N,1-dimethyl-N-(propan-2-yl)-1H-pyrazolo[3,4-d]pyrimidin-4-amine | C10 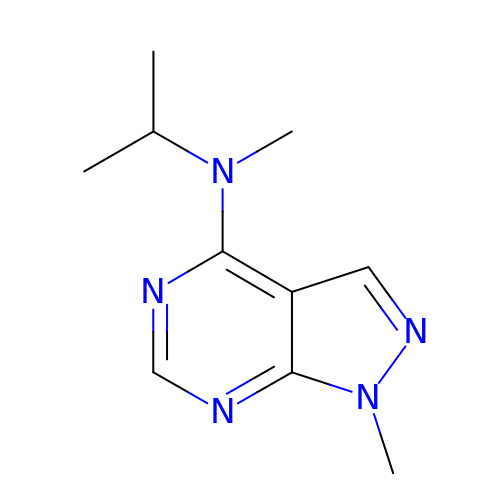H15 N5 | ACQZDWVVKAKBAO-UHFFFAOYSA-N> MAEPLLVVGLGNPGPTYAKTRHNLGFMVADVLAGRIGSAFKVHKKSGAEVVTGRLAGTTVVLAKPRISMNESGRQVGPLAKFYSVPPQQIVVIHDELD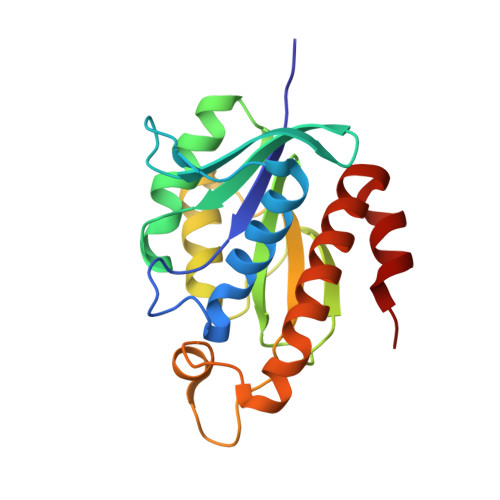IDFGRIRLKLGGGEGGHNGLRSVASALGTKNFHRVRIGVGRPPGRKDPAAFVLENFTSAERAEVPTIVEQAADATELLIAQGLEPAQNTVHAW>[2x]MGKGDVNVTSNVQAITSPQTTTIDNQTGAVTYSNWDGKVNGTVTATYNGQSYTATLNETAGKENSRVTPWYTQDGGKTWNVLKKDGGVYRLEPAGKYQLSVNNVSFNFGTANANKKNITLTSSNGVQFRENGQWKDSIKVSTDQNGAVSQPLTLLIPITPVDVTNAKSHHHHHH

S-layer proteins (SLPs) are self-assembling, crystalline proteins coating the cell surfaces of many prokaryotes. We determined the atomic resolution structures of all functional domains (I-III from N- to C-termini) present in the three S-layer proteins SlpA_ac, SlpX_ac, and SlpA_amy. The Lactobacillus S-layers are anchored to the cell wall through interaction with teichoic acids (TA), either lipoteichoic acid (LTA) or wall teichoic acid (WTA).

The arrangement and architecture of SlpA_ac and SlpA_amy are highly similar. The N-terminal part, exhibiting the first two domains (SlpA_I and SlpA_II), is known to be responsible for the self-assembly of the S-layer protein into a regular lattice. The crystal structures of SlpA from L. acidophilus and L. amylovorus and observed crystal contacts reveal the self-assembly formation. A second interaction was observed within this crystal structure, a symmetrical homodimer interaction spanning from Asn92 to Asn176. The self-assembly region (SA) is formed by domains SlpA_I and SlpA_II, building a 2D crystalline network that forms the exposed surface of the SlpA layer.> GPLAFCGSENHSAAYRVDQGVLNNGCFVDALNVVPHVFLLFITFPILFIGWGSQSSKVHIHHSTWLHFPGHNLRWILTFMLLFVLVCEIAEGILSDGVTESHHLHLYMPAGMAFMAAVTSVVYYHNIETSNFPKLLIALLVYWTLAFITKTIKFVKFLDHAIGFSQLRFCLTGLLVILYGMLLLVEVNVIRVRRYIFFKTPREVKPPEDLQDLGVRFLQPFVNLLSKGTYWWMNAFIKTAHKKPIDLRAIGKLPIAMRALTNYQRLCEAFDAQVRKDIQGTQGARAIWQALSHAFGRRLVLSSTFRILADLLGFAGPLCIFGIVDHLGKENDVFQPKTQFLGVYFVSSQEFLANAYVLAVLLFLALLLQRTFLQASYYVAIETGINLRGAIQTKIYNKIMHLSTSNLSMGEMTAGQICNLVAIDTNQLMWFFFLCPNLWAMPVQIIVGVILLYYILGVSALIGAAVIILLAPVQYFVATKLSQAQRSTLEYSNERLKQTNEMLRGIKLLKLYAWENIFRTRVETTRRKEMTSLRAFAIYTSISIFMNTAIPIAAVLITFVGHVSFFKEADFSPSVAFASLSLFHILVTPLFLLSSVVRSTVKALVSVQKLSEFLSSAEIREEQCAPHEPTPQGPASKYQAVPLRVVNRKRPAREDCRGLTGPLQSLVPSADGDADNCCVQIMGGYFTWTPDGIPTLSNITIRIPRGQLT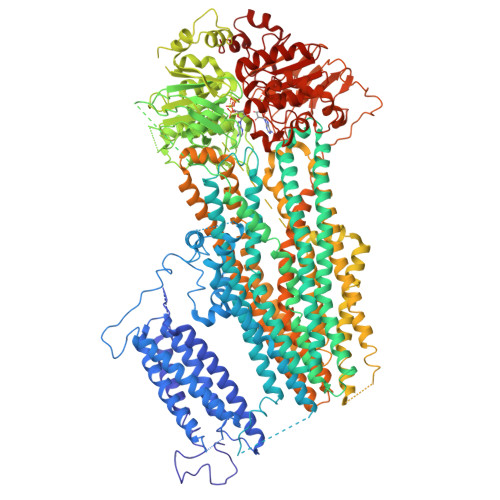MIVGQVGCGKSSLLLAALGEMQKVSGAVFWSSLPDSEIGEDPSPERETATDLDIRKRGPVAYASQKPWLLNATVEENIIFESPFNKQRYKMVIEACSLQPDIDILPHGDQTQIGERGINLSGGQRQRISVARALYQHANVVFLDDPFSALDIHLSDHLMQAGILELLRDDKRTVVLVTHKLQYLPHADWIIAMKDGTIQREGTLKDFQRSECQLFEHWKTLMNRQDQELEKETVTERKATEPPQGLSRAMSSRDGLLQDEEEEEEEAAESEEDDNLSSMLHQRAEIPWRACAKYLSSAGILLLSLLVFSQLLKHMVLVAIDYWLAKWTDSALTLTPAARNCSLSQECTLDQTVYAMVFTVLCSLGIVLCLVTSVTVEWTGLKVAKRLHRSLLNRIILAPMRFFETTPLGSILNRFSSDCNTIDQHIPSTLECLSRSTLLCVSALAVISYVTPVFLVALLPLAIVCYFIQKYFRVASRDLQQLDDTTQLPLLSHFAETVEGLTTIRAFRYEARFQQKLLEYTDSNNIASLFLTAANRWLEVRMEYIGACVVLIAAVTSISNSLHRELSAGLVGLGLTYALMVSNYLNWMVRNLADMELQLGAVKRIHGLLKTEAESYEGLLAPSLIPKNWPDQGKIQIQNLSVRYDSSLKPVLKHVNALIAPGQKIGICGRTGSGKSSFSLAFFRMVDTFEGHIIIDGIDIAKLPLHTLRSRLSIILQDPVLFSGTIRFNLDPERKCSDSTLWEALEIAQLKLVVKALPGGLDAIITEGGENFSQGQRQLFCLARAFVRKTSIFIMDEATASIDMATENILQKVVMTAFADRTVVTIAHRVHTILSADLVIVLKRGAILEFDKPEKLLSRKDSVFASFVRADK> GPGMAVKHLIVLKFKDEITEAQKEEFFKTYVNLVNIIPAMKDVYWGKDVTQKN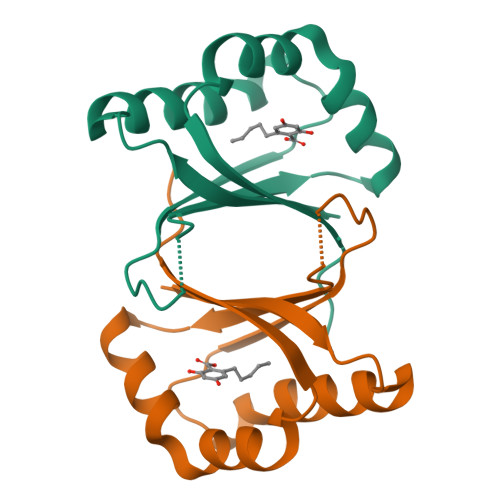KEEGYTHIVEVTFESVETIQDYIIHPAHVGFGDVYRSFWEKLLIFDYTPRK> AGKKPKQATLARFFTSMK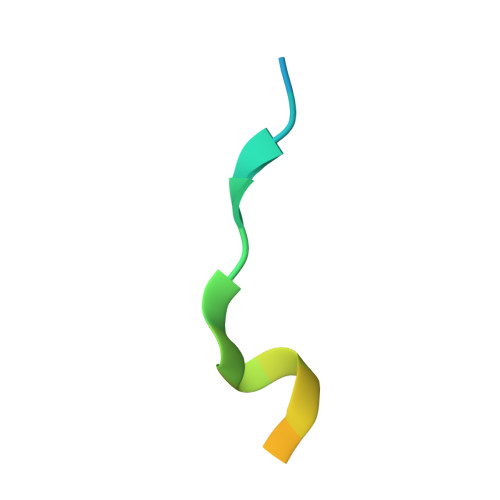NKPT2,2-dimethylpropyl (1S)-1-methyl-8-[(7-methyl-1H-indazol-5-yl)carbonyl]-2,8-diazaspiro[4.5]decane-2-carboxylate | C24 H34 N4 O3 | 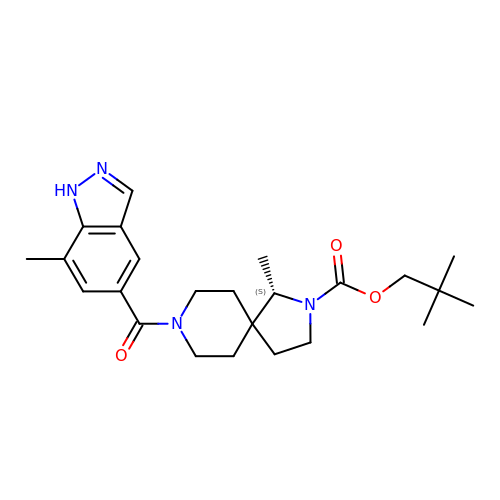ZOGULHIZBGRKQX-KRWDZBQOSA-N>[2x]MSTPHTDFFGLTIPFMQLLGVVPEHSGNGTARTRLPARADLVNSRGDIHGGTLMSVLD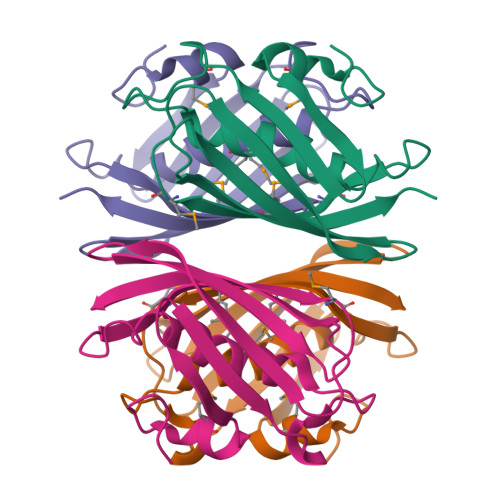FTLGAAIRGDTPEVGVATIDMNTSFMSPGRGDLVIETRCLRRGASIAFCEGEIRDSAGELVAKATATFKIIQRRPGLEHHHHHH> MGTKIIINVIFFDIILALLMMSFASIQPPSIANPPT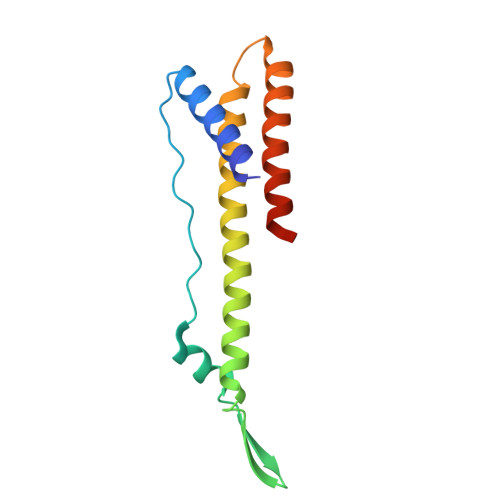VAQAQAQANITWNLTVGSINWEWLWPVFYFVDWLIWIVTTIFAVVAFIFNVFTTSLSLLASVPIVGPFLLMFAVIINFVLIWEVVKLIRGYDNPG>[2x]GANRTLIVTTILEEPYVMYRKSDKPLYGNDRFEGYCLDLLKELSNILGFLYDVKLVPDGKYGAQNDKGEWNGMVKELIDHRADLAVAPLTITYVREKVIDFSKPFMTLGISILYRKGTPIDSADDLAKQ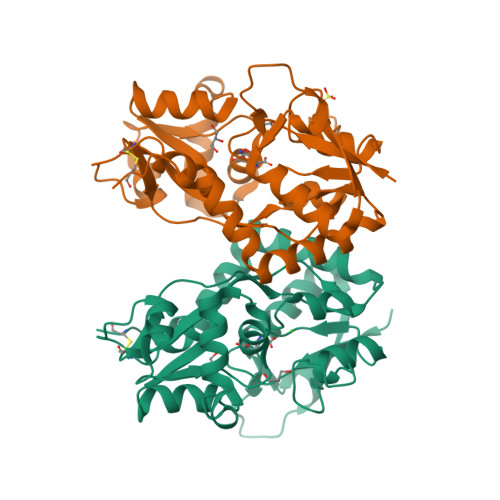TKIEYGAVRDGSTMTFFKKSKISTYEKMWAFMSSRQQSALVKNSDEGIQRVLTTDYALLMESTSIEYVTQRNCNLTQIGGLIDSKGYGVGTPIGSPYRDKITIAILQLQEEGKLHMMKEKWWRGNGCP CRYSTAL VIOLET | C25 H30 N3 | 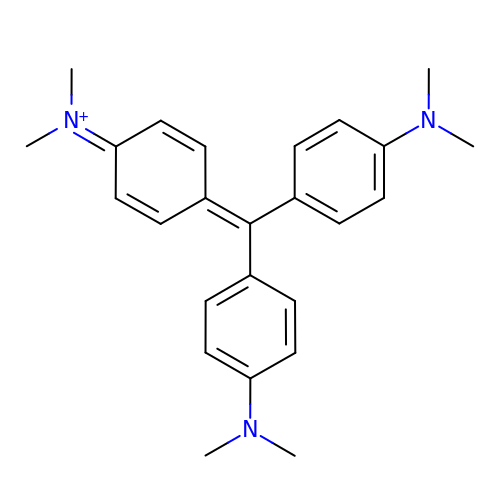LGLFFNDHMLKUMI-UHFFFAOYSA-N> MNLPTAQEVQGLMARYIELVDVGDIEAIVQMYADDATVENPFGQPPIHGREQIAAFYRQGLGGGKVRACLTGPVRASHNGC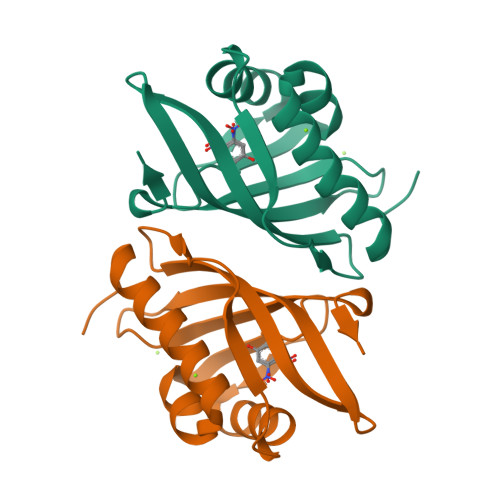GAMPFRVEMVWNGQPCALDVINVMRFDEHGRIQTMQAYWSEVNLSVREPQ>MHHHHHHHHGGSEFSIDGGSLEVLFQGPSSPPDLPVAISLRSFARILPDGDPKAVYGMVRALIMQLAAFHSPDDVRITVCASRERMPQWQWMKWLPHSLHPTEYDAAGQVRLLTHSLVELESMLGPEIKDRGMFGASRAPAEPFHLVIVDGGQASYDSQIASDGIDGVCVIDLTGSVAETNEATMLRLRVTPERVYVVKRDRAGKEVLSSVGRPDQASIAEAEALARQLAPFRTSAADEPEEDVLSANMTLTSLLHIDNPYNLDPAVLWRPRPQRNRLRVPIGLDADGRPLELDIKESAQGGMGPHGLCIGATGSGKSELLRTLVLALAMTHSPEVLNFVLVDFKGGATFLGMEGLRHVSAIITNLEEELPLVDRMYDALHGEMVRRQEHLRHSGNYASLRDYEKARMEGAPLPPMPTLFIVLDEFSELLSAKPDFAELFVMIGRLGRSLGVHLLLASQ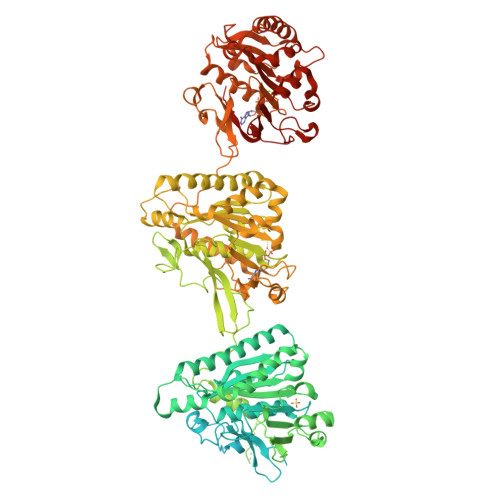RLEEGKLRGLDTHLSYRIGLRTFSAMESRVVLGVPDAYELPPSPGNGYLKFATEPLVRFKAAYVSGPVDEEPQTRSEGPQIVRQVLPYLTDYIRPQVVEQPQPEQRAEENKSSESLFDVVVRQLAGHGPEPHQIWLPPLDVPPTLDELLPPLSPSAAHGYTADGWEWRGRLHAVVGLVDRPFDQRRDPYWLDLSGGAGHVGVAGGPQTGKSTMLRTLITSLALLHTPQEVQFYCLDFGGGTLAGLAELPHVGSVATRLDADRIRRTVAEVSALLEQREQEFTERGIDSMATYRRLRATGEYAGDGFGDVFLVVDNWLTLRQDYEALEDSITQLAARGLGYGIHVVLSSNKWSEFRTSIRDLLGTKLELRLGDPYESEVDRKKAANVPENRPGRGLTRDGYHFLTALPRIDGDTSAETLTEGIATTVKTIREAWHGPTAPPVRMLPNVLPAAQLPSAAESGTRIPIGIDEDSLSPVYLDFNTDPHFLVFGDTECGKSNLLRLITAGIIERYTPQQARLIFIDYSRSLLDVATTEHQIGYAASSTAASSLVRDIKGAMEARLPPPDLTPEQLRSRSWWTGAELFLVVDDYEMVATSDNPLRPLAELLPQARDIGLHLIIARSMGGAGRALYEPIIQRIKEMASPGLVMSGNKDEGILLGNVKPHKLPQGRGYFVERRSGTRLIQTAYRES[2x]> VVGGEDARPNSWPWQVSLQYDSSGQWRHTCGGTLVDQSWVLTAAHC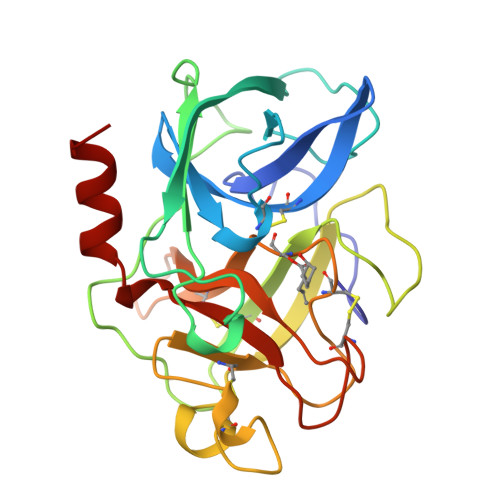ISSSRTYRVVLGRHSLSTNEPGSLAVKVSKLVVHQDWNSNQLSNGNDIALLKLASPVSLTDKIQLGCLPAAGTILPNNYVCYVTGWGRLQTNGASPDILQQGQLLVVDYATCSKPGWWGSTVKTNMICAGGDGIISSCNGDSGGPLNCQGANGQWQVHGIVSFGSSLGCNYYHKPSVFTRVSNYIDWINSVIANN> FGNWT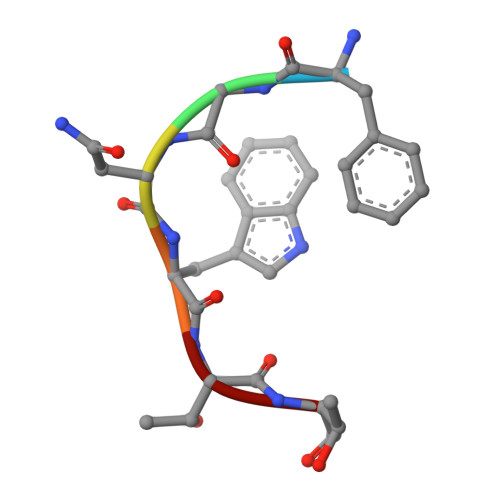T> GPLGSALEIAEQLTLLDHLVFKSIPYEEFFGQGWMKAEKYERTPYIMKTTKHFNHVSNFIASEIIRNEDISARASAIEKWVAVADICRCLHNYNAVLEITSSINRSAIFRLK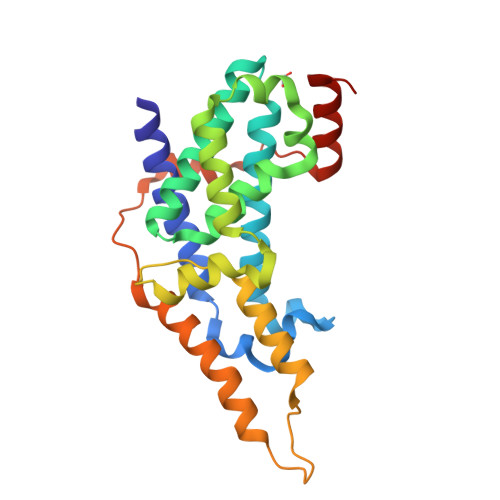KTWLKVSKQTKSLLDKLQKLVSSDGRFKNLRESLRNCDPPCVPYLGMYLTDLVFIEEGTPNYTEDGLVNFSKMRMISHIIREIRQFQQTTYKIDPQPKVIQYLLDESFMLDEESLYESSLLIEPKLPT>FSNLAIYWGQGPNQLRLSHFCQETSLDIINIGFINYFPDMSPGHWPGSNFGNQCDGSVYVTNDGVVTKLLSGCHQIMEDIPICQAAGKKVLLSIGGAYPPDQSILSEDSAVAFATFLWGAFGPVAEGWEGPRPFGDVVVDGFDFDIEHNGGFGYATMVNTFRQYFNQVPERKFYLSAAPQCIIPDAQLSDAIFNAAFDFIWIQYYNTAACSAKSFIDTSLGTFNFDAWVTVLKASASKDAKLYVG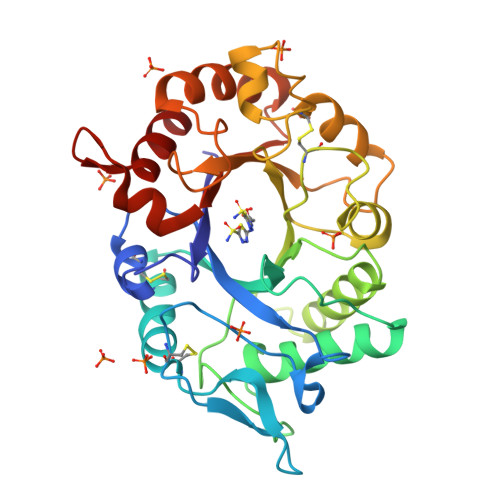LPASETAANQGYYLTPDEVESLVSTYMDRYPDTFGGIMLWEATASENNQIDGAPYADHMKDILLH[2x]4,4'-methylenediphenol 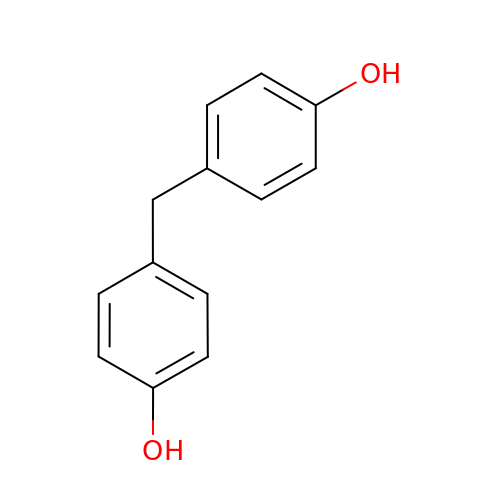| C13 H12 O2 | PXKLMJQFEQBVLD-UHFFFAOYSA-N>MASSVGNVADSTEPTKRMLSFQGPMELAHREYQAGDFEAAERHCMQLWRQEPDNTGVLLLLSSIHFECRRLDRSAHFSTLAIKQNPLLAEAYSNLGNVYKERGQLQEAIEHYRHALRLKPDFIDGYINLAAALVAAGDMEGAVQAYVSALQYNPDLYCVRSDLGNLLKALGRLEEAKACYLKAIETQPNFAVAWSNLGCVFNAQGEIWLAIHHFEKAVTLDPNFLDAYINLGNVLKEARIFDRAVAAYLRALSLSPNHAVVHGNLACVYYEQGLIDLAIDTYRRAIELQPHFPDAYCNLANALKEKGSVAEAEDCYNTALRLCPTHADSLNNLANIKREQGNIEEAVRLYRKALEVFPEFAAAHSNLASVLQQQGKLQEALMHYKEAIRISPTFADAYSNMGNTLKEMQDVQGALQCYTRAIQINPAFADAHSNLASIHKDSGNIPEAIASYRTALKLKPDFPDAYCNLAHCLQIVCDWTDYDERMKKLVSIVADQLEKNRLPSVHPHHSMLYPLSHGFRKAIAERHGNLCLDKINVLHKPPYEHPKDLKLSDGRLRVGYVSSDFGNHPTSHLMQSIPGMHNPDKFEVFCYALSPDDGTNFRVKVMAEANHFIDLSQIPCNGKAADRIHQDGIHILVNMNGYTKGARNELFALRPAPIQAMWLGYPGTSGALFMDYIITDQETSPAEVAEQYSEKLAYMPHTFFIGDHANMFPHLKKKAVIDFKSNGHIYDNRIVLNGIDLKAFLDSLPDVKIVKMKCPDGGDNADSSNTALNMPVIPMNTIAEAVIEMINRGQIQITINGFSISNGLATTQINNKAATGEEVPRTIIVTTRSQYGLPEDAIVYCNFNQLYKIDPSTLQMWANILKRVPNSVLWLLRFPAVGEPNIQQYAQNMGLPQNRIIFSPVAPKEEHVRRGQLADVCLDTPLCNGHTTGMDVLWAGTPMVTMPGETLASRVAASQLTCLGCLELIAKNRQEYEDIAVKLGTDLEYLKKVRGKVWKQRISSPLFNTKQYTMELERLYLQMWEHYAAGNKPDHMIKPVEVTESAHHHHHH[2x]

A single pair of enzymes, the O-GlcNAc transferase (OGT) and O-GlcNAcase (OGA), catalyzes the addition and removal of O-GlcNAc on over 3,000 proteins in the human proteome. OGT contains an N-terminal tetratricopeptide repeat (TPR) domain required for substrate recognition and a C-terminal glycosyltransferase family B domain (GTD) that catalyzes the modification of protein substrates with uridine diphosphate GlcNAc (UDP-GlcNAc) as the sugar donor. Here, we present the cryo-electron microscopy (cryo-EM) structures of human OGT and the OGT-OGA complex. Conversely, OGT disrupts the functional dimerization of OGA and occludes its active site, resulting in the blocking of access by other substrates. This mutual inhibition between OGT and OGA may limit the futile O-GlcNAcylation cycles and help to maintain O-GlcNAc homeostasis.

We next determined the structure of OGT at an overall resolution of 3.69 Å using single-particle cryo-EM. As previously reported, OGT formed a scissor-shaped dimer. The TPR domain of each monomer consists of 27 antiparallel α-helices, which stack together in a right-handed superhelical conformation with a lumen of 22 Å in diameter. The conserved asparagine residues line along the lumen and align in a ladder-like configuration to engage substrates. Structural comparison with previously solved OGT structures reveals that the catalytic domain (GTD477–1046) in all structures adopts an almost identical conformation. Consistent with earlier studies, TPR6 and TPR7 of OGT mediate its dimerization. Mutations of four conserved residues at the dimer interface to alanine (OGT 4A, W208A/L209A/I211A/H212A) disrupted OGT dimerization, based on size exclusion chromatography and cryo-EM analysis. Similar to the previous reports that showed the dimerization-defective OGT exhibited lower O-GlcNAc transferase activity towards substrates, here OGT 4A mutant was less active in catalyzing O-GlcNAcylation of both TAB1 and YTHDF1 here in vitro, indicating that OGT dimerization promotes optimal modification of certain substrates. We hypothesize that the dimerization of OGT stabilizes the mid-sections of the two α-solenoids in the dimer, allowing each solenoid to transiently reach its more straightened conformation for substrate recruitment and release.>TQGVITWDPYEYNAQNTTLYTKDLRDSFKEVRYNIWRTADGPESKQTFTSQEKDRDFALPLHLKTFHLKRGEFQI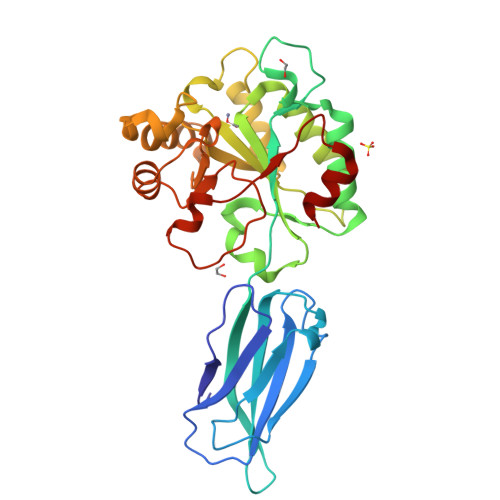ETVGIKEDNTETNLVTSKITFQQHVPVLMYHAIEKFPGPSDGDYGLYVPPEQFEKHMQYLKDNGYTMLTFERWNDINRVNKPIFITMDDGRKNNMNALHILQKLKDDTFQPAATEFLTANEIDKPNRLSTDDIKQMMDSGIFSIQSHTANHTMMAHSNNYDEELRGSKEKIEALTGKKVIALAYPVGSYNDPAVEETKKYYEFAVTTDHGNHITKGMPNEQYLIKRHFVGPNTSMEKFISLIK[2x]> MENTENSVDSKSIKNLEPKIIHGSESMDSGISLDNSYKMDYPEMGLCIIINNKNFHKSTGMTSRSGTDVDAANLRETFRNLKYEVRNKNDLTREEIVELMRDVSKEDHSKRSSFVCVLLSHGEAGIIFGTNGPVDLKKITNFFRGDRCRSLTGKPKLFIIQACRGTELDCGIETDSGVDDDMACHKIPVEADFLYACS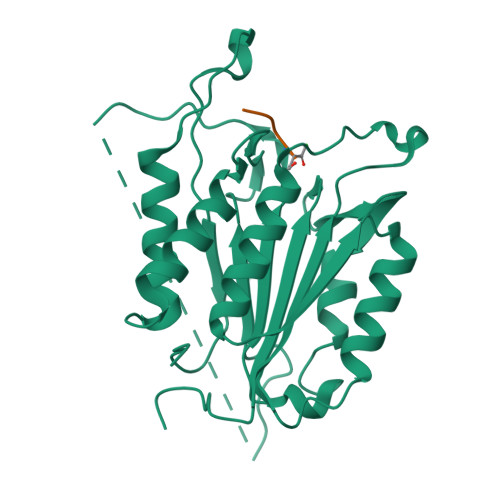TAPGYYSWRNSKDGSWFIQSLCAMLKQYADKLEFMHILTRVNRKVATEFESFSFDATFHAKKQIPCIHSMLTKELYFYH Here, we report the crystal structures of PstA from L. monocytogenes (LmPstA) bound to c-di-AMP and in the apo form. On the basis of these observations, we conclude that PstA is related to the larger PII protein superfamily, but has diverged through evolution to specifically recognize the bacterial second messenger c-di-AMP and thus is structurally and functionally distinct from the canonical PII proteins. The structure of each LmPstA monomer is composed of a four-stranded antiparallel β-sheet packed against two α-helices on one face. In the LmPstA trimer, the β-sheet of the three monomers form the core, and the α-helices are on the periphery.

We cocrystallized LmPstA with c-di-AMP and determined the structure of the complex at 1.6 Å resolution by the molecular replacement method. Three c-di-AMP molecules are bound to symmetrically equivalent locations on the LmPstA homotrimer, located in the inter-subunit cleft between β1 and β4, and the T/B-loops of one monomer and α1, β2–β3, and β5 of a neighboring monomer. The adenine base of the first nucleotide of c-di-AMP is recognized specifically by LmPstA, through hydrogen-bonds between its N1 and N6 atoms with the main chain amide and carbonyl of Gly47 (at the end of β3), respectively. The phosphate group is hydrogen-bonded to the side chain His108 (β5) and the main chain amide of Gly94 (B-loop of neighboring molecule). In contrast the recognition of the second nucleotide of the c-di-AMP molecule is mediated by unique structural features in PstA, due primarily to the significant structural differences in the T-loop which forms a part of the inter-subunit cleft where the ligand binds. Instead, the T-loop in PstA forms a shorter, more structured loop with a conserved 34-GGFL-37 sequence in the turn. The main chain amides of Gly35, Phe36, and Leu37 have hydrogen-bonding interactions with the phosphate group of this nucleotide. The side chain of Phe36 is π-stacked against one face of the adenine, while its other face is exposed to the solvent. In comparison, the adenine base for the second nucleotide in two of the c-di-AMPs assumes a syn conformation while the third one has an anti conformation. In both conformations, the adenine base is π-stacked against the Phe36 side chain.

>[3x]MKLIFAIVQDQDSNRLSDALTKGNFGATKLATTGGFLKAGNTTFIIGTEDERVEDALAIIKENCKAREQMMTPSASLGVTVDTYVPYPIEVQVGGATVFVMPVESFHHFLEHH> MGHHHHHHMPMYEVQWKVVEESNGNNYSYIDPTQLPYDHKWEFPRNRLSFGKTLGAGAFGKVVEATAQGLIKSDAAMTVAVKMLKPSAHSTEREAL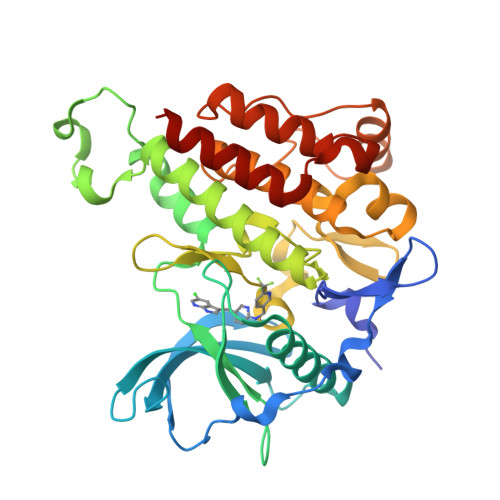MSELKVLSYLGNHENIVNLLGACTHGGPTLVITEYCCYGDLLNFLRRKRDSFHSSDTSPASMEDDENALDLEDLLSFSYQVAKGMAFLASKNCIHRDLAARNILLTHGRITKICDFGLARDIKNDSNYVDKGNARLPVKWMAPESIFNSVYTFESDVWSYGIFLWELFSLGSSPYPGMPVDSKFYKMIKEGFRMSSPEHAPAEMYDIMKTCWDADPDKRPTFKQIVQDIEKQISESTNH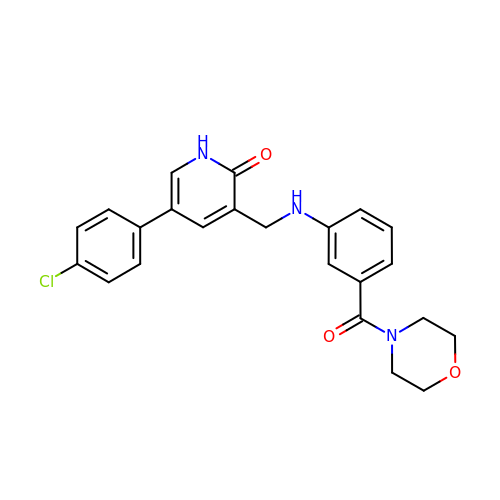5-(4-chlorophenyl)-3-({[3-(morpholine-4-carbonyl)phenyl]amino}methyl)pyridin-2(1H)-one | C23 H22 Cl N3 O3 | FGOXIGQZSJLIHW-UHFFFAOYSA-N> MSAGKLPEGWVIAPVSTVTTLIRGVTYKKEQAINYLKDDYLPLIRANNIQNGKFDTTDLVFVPKNLVKESQKISPEDIVIAMSSGSKSVVGKSAHQHLPFECSFGAFCGVLRPEKLIFSGFIAHFTKSSLYRNKISSLSAGANINNIKPASFDLINIPIPPLAEQKIIAEKLDTLLAQVDSTKARFEQIPQILKRFRQAVLGGAVNGKLTEKWRNFEPQHSVFKKLNFESILTELRNGLSSKPNESGVGHPILRISSVRAGHVDQNDIRFLECSESELNRHKLQDGDLLFTRYNGSLEFVGVCGLLKKLQHQNLLYPDKLIRARLTKDALPEYIEIFFSSPSARNAMMNCVKTTSGQKGISGKDIKSQVVLLPPVKEQAE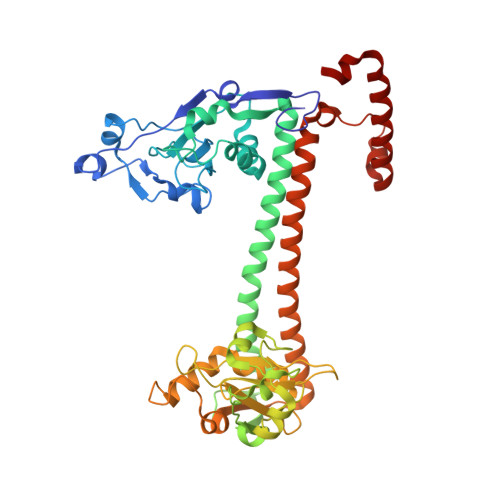IVRRVEQLFAYADTIEKQVNNALARVNNLTQSILAKAFRGELTAQWRAENPDLISGENSAAALLEKIKAERAASGGKKASRKKS> MQKINNINNNKQMLTRKEDLLTVLKQISALKYVSNLYEFLLATEKIVQTSELDTQFQEFLTTTIIASEQNLVENYKQKYNQPNFSQLTIKQVIDDSIILLGNKQNYVQQIGTTTIGFYVEYENINLSRQTLYSSNFRNLLNIFGEEDFKYFLIDFLVFTKVEQNGYLQVAGVCLNQYFSVQVKQKKWYKNNFNMNGKATSNNNQNNANLSNEKKQENQYIYPEIQRSQIFYCNHMGREPGVFKSSFFNYSEIKKGFQFKVIQEKLQGRQFINSDKIKPDHPQTIIKKTLLKEYQSKNFSCQEERDLFLEFTEKIVQNFHNINFNYLLKKFCKLPENYQSLKSQVKQIVQSENKANQQSCENLFNSLYDTEISYKQITNFLRQIIQNCVPNQLLGKKNFKVFLEKLYEFVQMKRFENQKVLDYICFMDVFDVEWFVDLKNQKFTQKRKYISDKRKILGDLIVFIINKIVIPVLRYNFYITEKHKEGSQIFYYRKPIWKLVSKLTIVKLEEENLEKVEEKLIPEDSFQKYPQGKLRIIPKKGSFRPIMTFLRKDKQKNIKLNLNQILMDSQLVFRNLKDMLGQKIGYSVFDNKQISEKFAQFIEKWKNKGRPQLYYVTLDIKKCYDSIDQMKLLNFFNQSDLIQDTYFINKYLLFQRNKRPLLQIQQTNNLNSAMEIEEEKINKKPFKMDNINFPYYFNLKERQIAYSLYDDDDQILQKGFKEIQSDDRPFIVINQDKPRCITKDIIHNHLKHISQYNVISFNKVKFRQKRGIPQGLNISGVLCSFYFGKLEEEYTQFLKNAEQVNGSINLLMRLTDDYLFISDSQQNALNLIVQLQNCANNNGFMFNDQKITTNFQFPQEDYNLEHFKISVQNECQWIGKSIDMNTLEIKSIQKQTQQEINQTINVAISIKNLKSQLKNKLRSLFLNQLIDYFNPNINSFEGLCRQLYHHSKATVMKFYPFMTKLFQIDLKKSKQYSVQYGKENTNENFLKDILYYTVEDVCKILCYLQFEDEINSNIKEIFKNLYSWIMWDIIVSYLKKKKQFKGYLNKLLQKIRKSRFFYLKEGCKSLQLILSQQKYQLNKKELEAIEFIDLNNLIQDIKTLIPKISAKSNQQNTN;> MKLTKGGSYILKKVDRKQFYQDEEIVMQIKKILGQKTTDCKQYIKCECIDGLGDEALIYFEMLANQNQHLQKNDVIMIQDYLNDKTQNDKIVVLVTRFQFCKASHVQPKTAQKESIQLLNTEKTIIQKSKITKNPAEEVLKFIEVNEKDNSSNSEDMIIEQQKQEIKNNQKEKQSINGFNLEDSYSNISDITNFGGKSNFNIGSLSDQLSKQTLLISQLQVGKNRFSFKFEGRVVYKSSTFQNQQDSKYFFITAQDANNQEINLSFWQKVDQSYQTLKVGQYYYFIGGEVKQFKNNLELKFKFGDYQIIPKETLSANYVQPLALQPSKQFGNDSIGDSDYSIHNLIEKEESIAQKGYNGQKNNKYRQNNNNSKHTLLISEVLKTSKQYLSVLAQVVDIQSSDKNIRLKICDNSCNQELKVVIFPDLCYEWRDKFSINKWYYFNEFVRQIYNDEVQLKNNIHSSIKESDDQRKVITYNQEQGVFKKSISINSNDSFEIKPKISYKNNSNQEQRIYSSIEEIIQQAQASEIGQKKEFYVYGNLVSIQMKNKLYYYRCTCQGKSVLKYHGDSFFCESCQQFINPQVHLMLRAFVQDSTGTIPVMIFDQQSSQLINQIDPSIHVQEAGQYVKNCIENGQEEIIRQLFSKLDFARFIFEIQFENKEFNNEQEIAYKVLKIEKENIKEESKYLLKKLEHLINNNQNN;> MSNRVQGGFDNNSGNNQSAQKQQAEKIPQITVPLNCFMINQIVKAAKENPQAHSGNHYEWYGAFENAIITAKFEFLQSINDSPKIMGKLSDSTGCIEVVIQKSKMSDELPEFVQAYEIELQNNGNRHKYVRAMLKMRKNAQIQLLYFSIVNDANEISRHG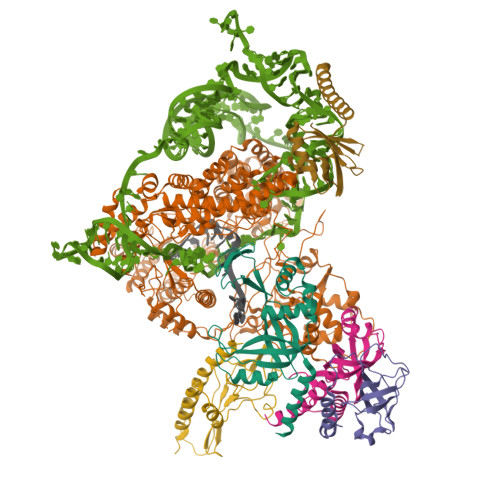LDLCLRYLQRKHGIEDFMHMTNDKAHNNHNASAQKVHYQIDRNQQPKEQVLELMRQILKHNPNDQIPKSKIIEFFQSQLNQVQINQILQQLVSANEIFSVGSDNYLLNV;> MDAEQEQVMYPRILFEQMAQFRGKKVTVVGNVCNEDQNDSLVIEFGPTGLNQHVVIDNYRRVDLNNTTKFVEIRGVVLNQNIVSCEELTEFEQKDPFDFDTYSKLIHLSQSDKLSSLFTDQ;> MDEYLENTNLEELEQECFMEDYQHEDVVEQENHQVDANDIYENQQMNDESQLNQDVKISQQKEQAVEMIEEQQQNNQDKFKQFQDCMAHITELNFKRNYQNLTEQSSSNNVVAEELDIKESLKLQMEYYFCDTNLTHDSYLRGIISKSPKNCVDIKVFLKFNKIQQILKQIQDKQIVSTYGIENQSQKKNHKNYKNQNATFSKKDLIHLIRDSLKESKILKVKMDSLKVKRRFPFNLEQALKNSKQRTLYIDFLPPKCSKQTLVSIFGNFRIININLPLQKNSQLCQGFAFIEFFSEEEANQALITKNSSIPKELILLTEKKIGQGSIRIITYKKWQEEKQSFKELSKNQNEQKNKNMNQSRKASDEFVSIDVEIKQNCLIKIINIPQGTLKAEVVLAVRHLGYEFYCDYIDENSNQINSNKISLSTQQQNTAQCSNIQIENNLIQQDQHPQLNDLLKEGQAMIRFQNSDEQRLAIQKLLNHNNNKLQIEIRGQICDVISTIPEDEEKNYWNYIKFKKNEFRKFFFMKKQQKKQNITQNYNK> AIGGPFQLTDQNGKAVTDKSLKGKPTLIFFGYTHCPDVCPTSLFEISEVLRAMGKDADKVNAIFISVDPERDTPATMKNYLSSFDPHLEGLSGDPAE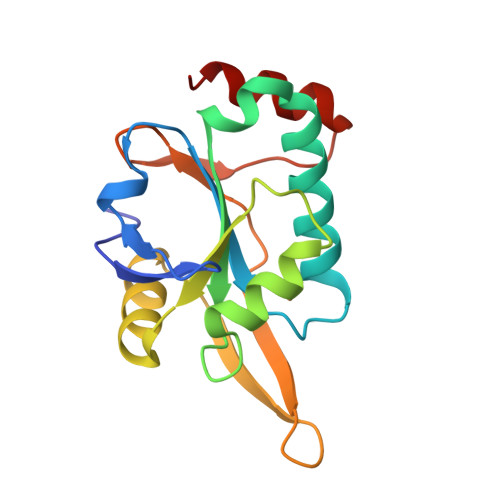IAKVITSYRVYAKKVPTKDGDYTMDHTALIYLMDRDGRFVSPFNLKRTPEEAAADLKRYL> MKTVLILAGLIALALSSTVPEFKTTPVDAAFVEKQKKILSLFYNVNEISYEAEYYKVAQDFNIEASKDCYTNMKAYENFMMMYKVGFLPKNLEFSIFYEKM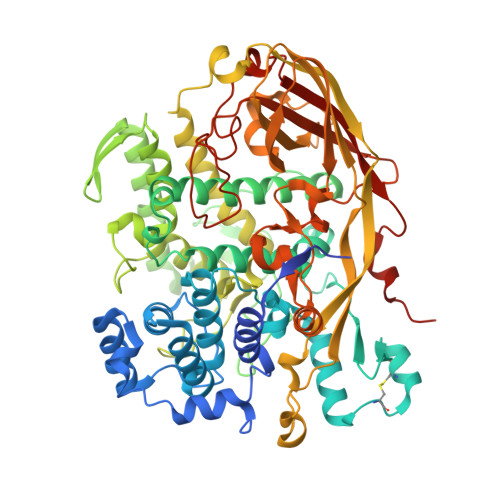REEAIALFKLFYYAKDFECFYKTACYARVYMNQGMFLYAYYIAIIQRSDTASFVLPAPYEAYPQYFVNMEVKNKMDYVKMMDGCLDEKICYNYGIIKENEQFVMYANYSNSLTYPNNEDRIAYLTEDVGLNAYYYYFHSHLPFWWNSGKYGAFKERRGEIYFFFYQQLLARYYMERLTNGLGKIPEFSWYSPLRTGYLPPFNSFYYPFAQRSNDYELHTEKNYEEIRFLDIYEKTFFQYLQQGHFKAFDKKIDLHSSKAVNFVGNYWQTNADLFEEDFLQFYQRSYEVNARRVLGAAPKPFNQYTFIPSALDFYQTSARDPAFYQLYKRIVQYIIEFKQYQVPYTQEALHFVGLKISDVKVDKMVTFFDHFDFDAFNTVYFSKEELKSSPHGYKVRQPRLNHKPFTVTIDIKSDVATNAVVKMFLGPKYDENGFPFSLEDNWMNFYELDWFVQKVNPGQSQITRSSTDFAFFKEDSLPMAEIYKLLDQGKIPTDMFNSSDTMPSRLMLPKGTYDGFPFQLFVFVYPYEPTPKESEPFKAVVPDNKPFGYPFDRPVLPQYFKQPNMFFKKVLVYHEGELFPYLFNIPHYTPDKAQL>[6x]VRSSSRTPSDKPVAHVVANPQAEGQLQWLNRRANALLANGVELRDNQLVVPSEGLYL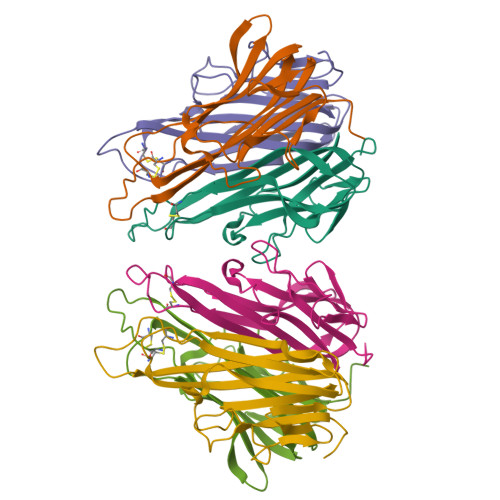IYSQVLFKGQGCPSTHVLLTHTISRIVVSYQTKVNLLSAIKSPCQRETPEGAEAKPWYEPIYLGGVFQLEKGDRLSAEINRPDYLLFAESGQVYFGIIAL>GSRATVFKLGLFKSLFLCSFHDITRLFKNDKTTNQQWVLAVFGLAEVFFEASFELLKKQCSFLQMQKRSHEGGTCAVYLICFNTAKSRETVRNLMANMLNVREECLMLQPPK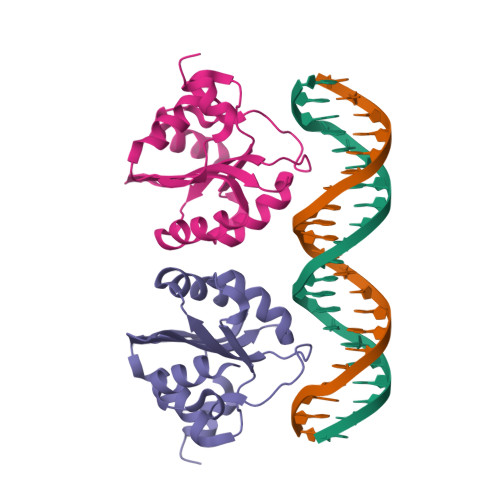IRGLSAALFWFKSSLSPATLKHGALPEWIRAQTTLNESLQTE[3x]>MVEIDPFEMAVKQLERAAQYMDISEEALEWLKKPMRIVEVSVPIEMDDGSVKVFTGFRVQHNWARGPTKGGIRWHPAETLSTVKALATWMTWKVAVVDLPYGGGKGGIIVNPKELSEREQERLARAYIRAVYDVIGPWTDIPAPDVYTNPKIMGWMMDEYETIMRRKGPAFGVITGKPLSIGGSLGRGTATAQGAIFTIREAAKALGIDLKGKKIAVQGYGNAGYYTAKLAKEQLGMTVVAVSDSRGGIYNPDGLDPDEVLKWKREHGSVKDFPGATNITNEELLELEVD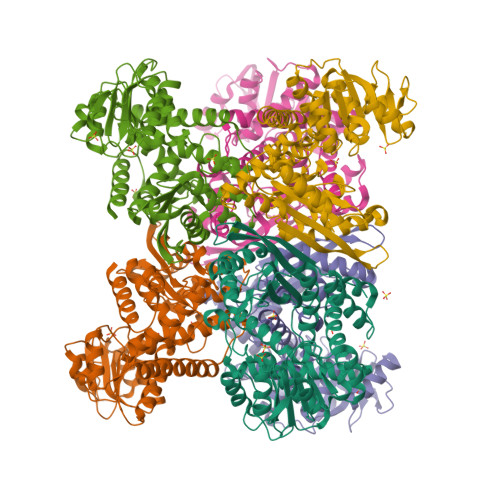VLAPAAIEEVITEKNADNIKAKIVAEVANGPVTPEADDILREKGILQIPDFLCNAGGVTVSYFEWVQNINGYYWTEEEVREKLDKKMTKAFWEVYNTHKDKNIHMRDAAYVVAVSRVYQAMKDRGWVKK[6x]>MVKLTAPKSNVVAYGNEFLKITATASDSDGKISRVDFLVDGEVIGSDREAPYEYEWKAVEGNHEISVIAYDDDDAASTPDSVKIFVKQARLEHHHHHH[4x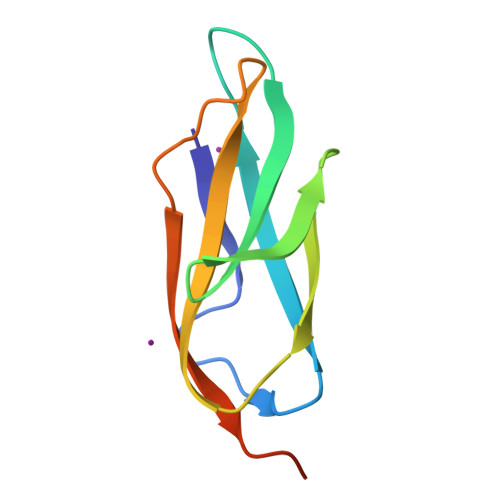]> AHMGCVSSKSTTVLSPQTSFNEASRTSFRALPGPSQRQLEVYDQCLIGAARWPDDSSKSNTPENRAYCQSMYNSIRSAGDEISRGGITSFEELWGRATEWRLSKLQRGEPLYSAFASERTSDTDAVTPLVKPYKSVLARVVDHEDAHDEIMQDNLFGDLNVKVYRQTAYLHGNVIPLNTFRVATDTEYLRDRVAHLRTELGAKALKQHLQRYNPDRIDHTNASYLPIIKDHLNDLYRQAISSDLSQAELISLIARTHWWAASAMPDQAGSAAKAEFAARAIASAHGIELPPFRNGNVSDIEAMLSGEEEFVEKYRSLLDSDCF

AvrB, a type III secretion system effector from the plant pathogen Pseudomonas syringae, is a member of the Fido (Fic, Doc, and AvrB) family that triggers HR in Arabidopsis plants to ward off systemic infection. Our investigations herein reveal the distinct and unexpected activity of AvrB acting as a glycosyltransferase that rhamnosylates residue T166 of Arabidopsis thaliana guardee protein RIN4. By elucidating the crystal structures of AvrB and its substrates across different enzymatic states, we provide an explanation for the specificity of substrates and delineate the step-by-step reaction mechanism executed by AvrB in the process of transferring rhamnose to RIN4. The identified biochemical activity of the avirulence protein AvrB as a rhamnosylator adds to the catalytic versatility of the Fido domain–containing protein superfamily.

Structures of AvrB + RIN4 [similar to a reported structure (19)], AvrB + RIN4 + UDP-rhamnose, AvrB + RIN4T166-Rha + UDP, and AvrBR266A + UDP together contribute to deciphering the catalytic mechanisms of AvrB as a rhamnosyltransferase. All the other four subfamilies of Fido domain–containing proteins use diphosphate nucleotide charged cosubstrates for catalytic reactions, and an ADP molecule could be soaked into the cosubstrate binding pocket of AvrB. Under the condition tested, ADP did not cause an obvious shift in the melting temperature, while UDP caused an obvious shift (~+0.8°C). Thus, UDP appears to be the nucleotide capable of binding to AvrB and may be part of the cosubstrate used by AvrB. AvrBG46D and AvrBY65A both caused a +146-Da mass increase in RIN4; however, coexpression with mutants of potential catalytic residues, AvrBR266A or AvrBD297A, did not induce a mass shift. When RfbA, RfbB, RfbC, and RfbD were coexpressed with WT AvrB, but not the R266A mutant, we observed RIN4 rhamnosylation.>GVTVIPRLLGLKDEKKIATTVGEARLSGINYRHPDSALVSYPVAAAAPLGRLPAGNYRIAIVGGGAGGIAALYELGRLAATLPAGSGIDVQIYEADPDSFLHDRPGIKAIKVRGLKAGRVSAALVHNGDPASGDTIYEVGAMRFPEIAGLTWHYASAAFGDAAPIKVFPNPGKVPTEFVFGNRVDRYVGSDPKDWEDPDSPTLKVLGVVAGGLVGNPQGENVAMYPIANVDPAKIAAILNAATPPADALERIQTKYWPEFIAQYDGLTLGAAVREIVTVAFEKGTLPPVDGVLDVDESISYYVELFGRFGFGTGGFKPLYNISLVEMMRLILWDYSNEYTLPVTENVEFIRNLFLKAQNVGAGKLVVQVRQERVANACHSGTASARAQLLSYDSHNAVHSEAYDFVILAVPHDQLTPIVSRSGFEHAASQNLGDAGLGLETHTYNQVYPPLLLSDSSPAANARIVTAIGQLHMARSSKVFATVKTAALDQPWVPQWRGEPIKAVVSDSGLAASYVVPSPIVEDGQAPEYSSLLASYTWEDDSTRLRHDFGLYPQNPATETGTADGMYRTMVNRAYRYVKYAGASNAQPWWFYQLLAEARTADRFVFDWTTNKTAGGFKLDMTGDHHQSNLCFRYHTHALAASLDNRFFIASDSYSHLGGWLEGAFMSALNAVAGLIVRANRGDVS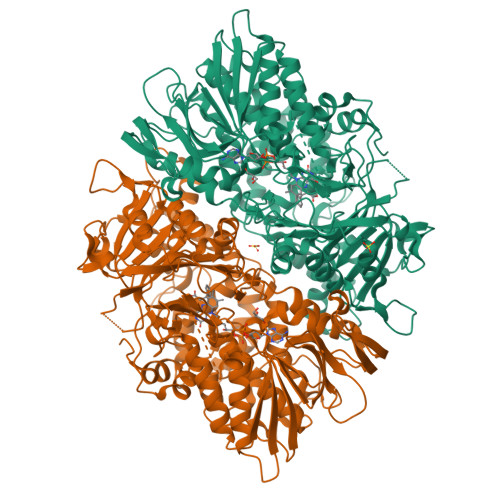ALSTEARPLVIGLRPVVKVPAAELATSQLEHHHHHH[2x]>MSGNEKHKENVAIENDGTPPRDKESLSPLTRFLNNELYGEKDARRKIGEITQTLLDHAVENGESQKVTLKGEVGRLTGYYHQGAASSEGETSATSGKVVLFLHGSGSSAEEQASEIRNHYQKQGIDMLAVNLRGYGESDGGPSEKGLYQDARTMFNYLVNDKGIDPSNIIIHGYSMGGPIAADLARYAAQNGQAVSGLLLDRPMPSMTKAITAHEVANPAGIVGAIAKAVNGQFSVEKNLKGLPKETPILLLTDNEGLGEEGEKLRAKLAIAGYNVTGEQTFYGHEASNRLMGQYADQIVSGLFNAEQAAVEAGEVLKGLEKDFKRYGDALKPDTSVPGKSKDIRTTKDFLNGYKNDHAKEIVDGFRSDMSIKQLVDLFVKGSWSAEQKGALAWEIESRALKVTFQNKSEKYNRLFREIASAGVVDAKATEQLAPQLMLLNLSNDGFGGRSDPLSKLVLVAKQLENDGQVGVARQLLEKMYSAAAVLSNPTLYSDSENANASKLLSSLAAIHAKNPMHDTSMKVWQEKLEGKQALTVNGVVEKITDASANGKPVLLELDAPGHAMAAWAKGSGDDRVYGFYDPNAGIVEFSSAEKFGDYLTRFFGKSDLNMA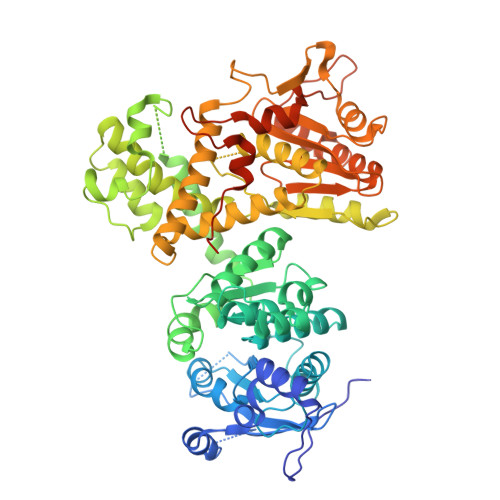QSYKLGKNDAGEAIFNRVVVMDGNTLASYKPTFGDKTTMQGILDLPVFDATPMKKPGTSDVDGNAKAVDDTKEALEHHHHHH[4x]[METHYLTELLURO]ACETATE | C3 H5 O2 Te | 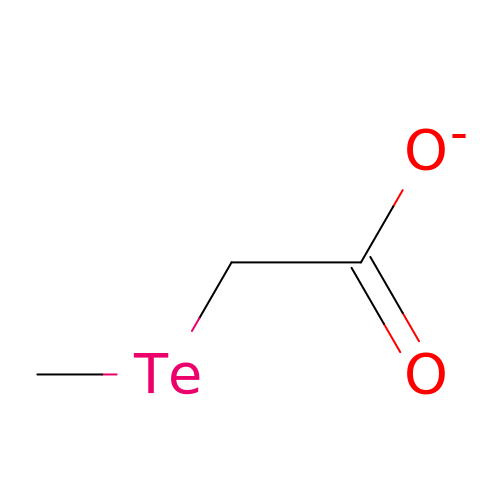OKJWQADPGUWQAJ-UHFFFAOYSA-M>MVKIVYPNAKDFFSFINSITNVTDSIILNFTEDGIFSRHLTEDKVLMAIMRIPKDVLSEYSIDSPTSVKLDVSSVKKILSKASSKKATIELTETDSGLKIIIRDEKSGAKSTIYIKAEKGQVEQLTEPKVNLAVNFTTDESVLNVIAADVTLVGEEMRISTEEDKIKIEAGEEGKRYVAFLMKDKPLKELSIDTSASSSYSAEMFKDAVKGLRGFSAPTMVSFGENLPMKIDVEAVSGGHMIFWIAPRL[2x];>MMKAKVIDAVSFSYILRTVGDFLSEANFIVTKEGIRVSGIDPSRVVFLDIFLPSSYFEGFEVSQEKEIIGFKLED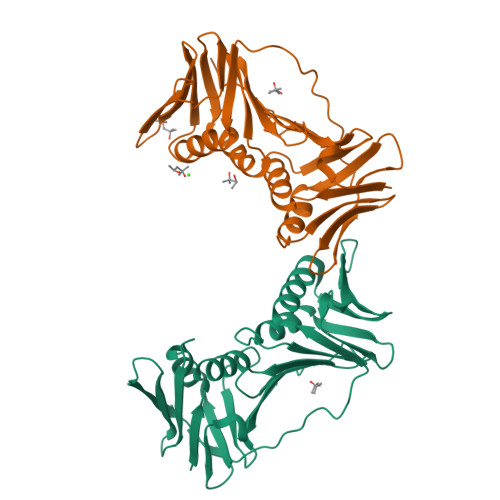VNDILKRVLKDDTLILSSNESKLTLTFDGEFTRSFELPLIQVESTQPPSVNLEFPFKAQLLTITFADIIDELSDLGEVLNIHSKENKLYFEVIGDLSTAKVELSTDNGTLLEASGADVSSSYGMEYVANTTKMRRASDSMELYFGSQIPLKLRFKLPQEGYGDFYIAPRAD[2x]>GPYMIQEEEWDRDLLLDPAWEKQQRKTFTAWCNSHLRKAGTQIENIEEDFRNGLKLMLLLEVISGERLPKPDRGKMRFHKIANVNKALDYIASKGVKLVSIGAEEIVDGNVKMTLGMIWTIILRFAIQDISVEETSAKEGLLLWCQRKTAPYRNVNIQNFHTSWKDGLGLCALIHRHRPDLIDYSKLNKDDPIGNINLAMEIAEKHLDIPKMLDAEDIVNTPKPD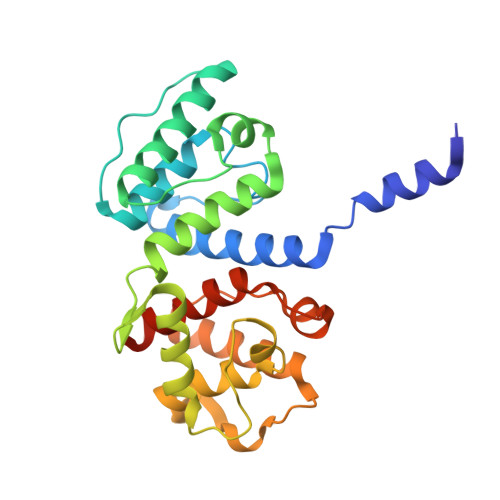ERAIMTYVSCFYHAFAGAEQAETAA[2x]Mitochondrial proteins CHCHD10 and CHCHD2 are mutated in rare cases of heritable FTD, ALS and PD and aggregate in tissues affected by these diseases. Here, we demonstrate that the low complexity N-terminal domains of both D10 and D2, as well as the full-length proteins, can form amyloid fibrils in vitro and in vivo. Structures of D10 and D2 fibrils assembled in vitro from the low complexity N-terminal domains of each protein show that their core comprises the most highly conserved region between the two proteins. For D10 and D2, the central conserved VAV motif forms a beta-strand that is associated with the protofilament interface in all the structures we have observed, suggesting that it may be a critical element in fibril formation and may be expected to appear in ex vivo structures as well.

Using cryo-EM, we observed several distinct D10-NT fibril polymorphs (see Methods section on Cryo-EM sample preparation and data collection) and determined three different structures. WT D10-NT polymorph-3, solved to 2.63 Å resolution, contains four identical PFs with yet a different fold (PF3) arranged as two helically symmetric dimers situated around a central pseudo-2-fold helical symmetry axis. PF3 is comprised of residues T50–G76 and contains only two beta strands consisting of T51–V57 and A68–V70, with an extensive turn between them. The central interface is quite small, consisting primarily of residues M65 and G66, while the PF interface within each symmetric dimer is extensive and comprises strand 1 and the first half of the turn between strands 1 and 2. However, in the PF2 and PF3 D10-NT folds, some of the sequence variation sites are positioned within the PF fold, suggesting that these D10-NT folds may not be compatible with the D2 sequence. Interestingly, residue S59 is a small sidechain that is packed inside the PF interior in all three wildtype (WT) D10-NT structures, while residues V57 and G58 are found either in the PF interior or at PF packing interfaces in all three D10-NT structures.

>[36x]MPRGSRSAASRPASRPAAPSAHPPAHPPPSAAAPAPAPSGQPGLMAQMATTAAGVAVGSAVGHVMGSALTGAFSGGSSEPSQPAVQQAPTPAAPQPLQ> VMGEDQQIPRNEAQHGVHPISIDTHRISNNWSPQAMCIGEKVVSIRQLIKRFGIFGDANTLQADGSSFVVAPFTVTSPTKTLTSTRNYTQFDYYYYLYAFWRGSMRIKMVAETQDGTGTPRKKTNFTWFVRMFNSLQDSFNSLISTSSSAVTTTVLPSGTINMGPSTQVIDPTVEGLIEVEVPYYNISHITPAVTIDDGTPSMEDYLKGHSPPCLLTFSPRDSISATNHIITASFMRALGDDFSFMYLLGVPPLVNVARA;> ENSHIENEDKRLTSEQKEIVHFVSEGVTPSTTALPDIVNLSTNYLDKNTREDRIHSIKDFLSRPIIIATNLWSVSDPVEKQLYTANFPEVLISNAMYQDKLKGFVGLRATLVVKVQVNSQPFQQGRLMLQYIPYAQYMPNRVTLINETLQGRSGCPRTDLELSVGTEVEMRIPYVSPHLYYNLITGQGSFGSIYVVVYSQLHDQVSGTGSIEYTVWAHLEDVDVQYPTGANIFTGNEAYIKGTSRYDAAQKAHAA;> SKPTVQGKIGECKLRGQGRMANFDGMDMSHKMALSSTNEIETNEGLAGTSLDVMDLSRVLSIPNYWDRFTWKTSDVINTVLWDNYVSPFKVKPYSATITDRFRCTHMGKVANAFTYWRGSMVY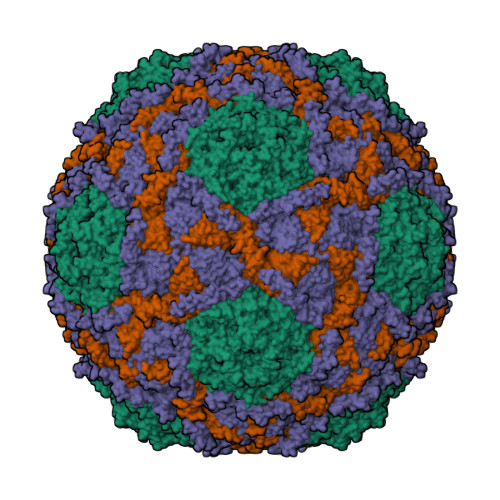TFKFVKTQYHSGRLRISFIPYYYNTTISTGTPDVSRTQKIVVDLRTSTAVSFTVPYIGSRPWLYCIRPESSWLSKDNTDGALMYNCVSGIVRVEVLNQLVAAQNVFSEIDVICEVNGGPDLEFAGPTCPRYVPYAGDFTLADTRKIEAERTQEYSNNED;> AASELKQLETNNSPSTALGQISEGLTTLSHIPVLGNIFSTPAWISAKAADLAKLFGF Recently we discovered a prokaryotic homolog of PepT1 from the bacterium Staphylococcus hominis, PepTSh, which was able to transport a natural thioalcohol-conjugated peptide, exhibiting structural characteristics similar to prodrug molecules. PepT1 and PepT2 belong to the much larger POT or PTR family of proton-coupled oligopeptide transporters, with homologs found in all domains of life except the archaea. POT family transporters belong to the major facilitator superfamily (MFS) of secondary active transporters, and use the proton electrochemical gradient to drive the concentrative uptake of di- and tripeptides into the cell. To address this question and understand how peptide-based prodrugs and nonproteinogenic drug molecules are recognized and transported via the SLC15 family, we determined the crystal structure of a bacterial POT family member in complex with both valacyclovir and 5-aminolevulinic acid at 3.1-Å and 2.5-Å resolution, respectively.

We successfully captured PepTSh in complex with 5-aminolevulinic acid and determined two structures at 2.5-Å and 2.8-Å resolution, respectively. Five-aminolevulinic acid is an endogenous nonprotein amino acid that forms the first part of the porphyrin synthesis pathway in mammals and is used in the clinic for the photo dynamic detection and treatment of cancer. PepTSh adopts an almost identical inward open state observed previously, with an rmsd of 0.305 Å over 480 Cα atoms compared with the valacyclovir structure. The 5-aminolevulinic acid molecule sits in a similar position as the l-valine scaffold in valacyclovir, adopting a vertical orientation. The C-terminal carboxyl group of 5-aminolevulinic acid faces toward the extracellular gate, making interactions with the backbone carbonyl group of Gln344 (Gln326) and via a water-mediated bridge to the side chain of this same residue. Five-aminolevulinic acid does not contain a peptide bond, having a ketomethylene group instead. This sits in close proximity to E418, in a similar position to the amino terminal group of the l-valine scaffold in valacyclovir. The amino terminal group in contrast sits in a similar position to the carboxyl group of valacyclovir, interacting with N167. Finally, during refinement it became clear that an unusual interaction could be observed within the binding site, wherein an arginine on TM1 (R37) and lysine on TM4 (K137) interact through a shared hydrogen bond. Of particular interest was the observation that 5-aminolevulinic acid adopted a vertical orientation as opposed to the horizontal one adopted by dipeptides in PepTSt.

> QTIQSIPQKGFFGHPRGLGVLFFVEFWERFSYYGMRAMLIFYMYFAIHQNGLGIDKTTAMSIMSVYGALIYMSSIPGAWIADRITGTRGATLLGAVLIIIGHICLSLPFALFGLFSSMFFIIIGSGLMKPNISNIVGRLYPENDTRIDAGFVIFYMSVNLGALISPIILQHFVDIRNFHGGFLLAAIGMALGLVWYLLFNRKNLGSVGMKPTNPLSKEEKRKYGMIIGIIVAIVIVVLLVTYYTHTLSFDLISNTVLVLGVALPIIYFTTMLRSKDVTDGERSRVKAFIPLFILGMLFWSIQEQGSNVLNIYGLERSDMQLNLFGWTTRFGEALFQSINPLFILLFAPVISMIWLKMGKKQPSLAIKFSIGTLLAGLSYILIGLVGLGYGHTQFSVNWVILSYVICVIGELCLSPTGNSAAVKLAPKAFNAQMMSVWLLTNASAQAINGTLVKLIKPLGQTNYFIFLGTVAIVITLIILVFSPKITK N-[(1R)-1-(3-chloro-4'-fluoro[1,1'-biphenyl]-4-yl)-2-(1H-imidazol-1-yl)ethyl]-4-{5-[3-fluoro-5-(5-fluoropyrimidin-4-yl)phenyl]-1,3,4-oxadiazol-2-yl}benzamide 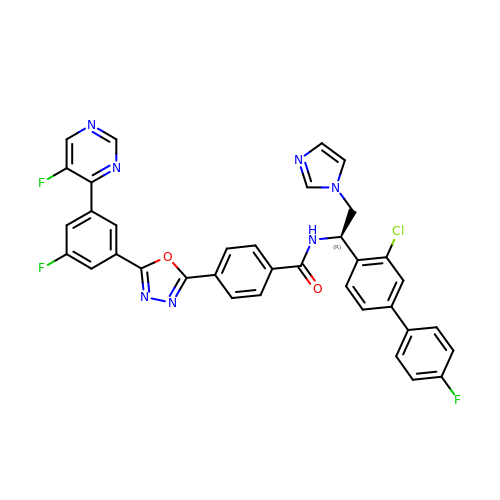| C36 H23 Cl F3 N7 O2 | ZSDQWZVUVIKSDR-YTTGMZPUSA-N>[2x]GMLHYTKEDLLELGAEITTREIYQQPDVWREAFEFYQAKREEIAAFLQE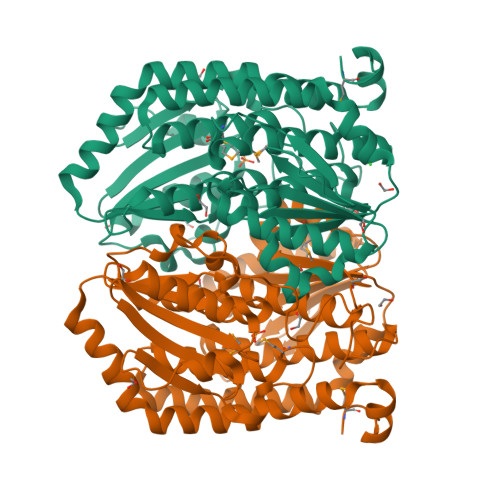IADKHDYIKVILTGAGTSAYVGDTLLPYFKEVYDERKWNFNAIATTDIVANPATYLKKDVATVLVSFARSGNSPESLATVDLAKSLVDELYQVTITCAADGKLALQAHGDDRNLLLLQPAVSNDAGFAMTSSFTSMMLTTLLVFDPTEFAVKSERFEVVSSLARKVLDKAEDVKELVDLDFNRVIYLGAGPFFGLAHEAQLKILELTAGQVATMYESPVGFRHGPKSLINDNTVVLVFGTTTDYTRKYDLDLVREVAGDQIARRVVLLSDQAFGLENVKEVALGCGGVLNDIYRVFPYIVYAQLFALLTSLKVENKPDTPSPTGTVNRVVQGVIIHEYQK>MSDNDELQQIAHLRREYTKGGLRRRDLPADPLTLFERWLSQACEAKLADPTAMVVATVDEHGQPYQRIVLLIHYDEKGMVFYTNLGSRKAHQIENNPRVSLLFPWHTLERQVMVIGKAERLSTLEVMKFFHSLPRDSQIGAWVSKQSSRISARGILESKFLELKQKFQQGEVPLPSFWGGFRVSLEQIEFWQGGEHRLADRFL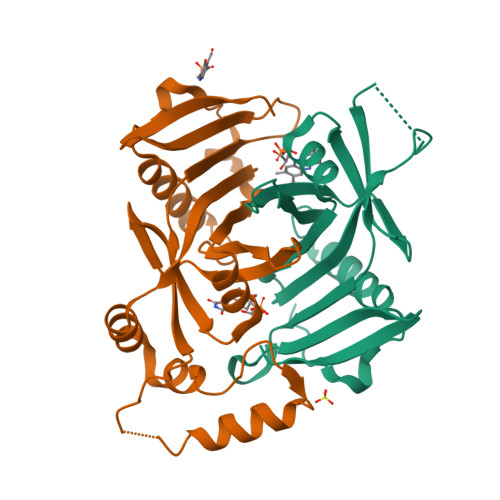YQRENDAWKIDRLAP[2x]>MSLSIPTIKQVRAFVLRGGGADYHDQGDGHWIDDHISTPMGKYPEYRQSRRSFGINVLGTLVVEIEASDGNVGFAVTTGGEPAAYIVEKHLARFLEGARVTDIER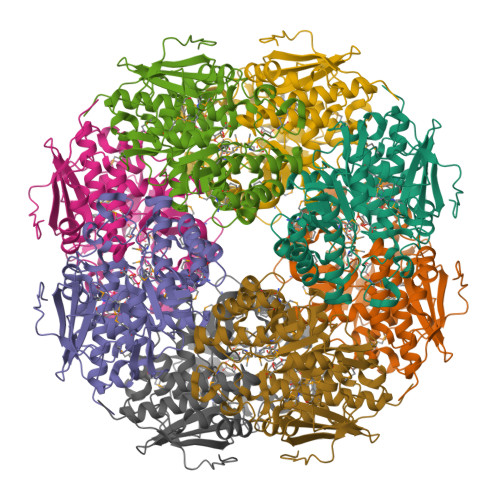IWDQMYNSTLYYGRKGLVINTISGVDLALWDLLGKVRREPVHQLLGGAVRDELQFYATGARPDLAQKMGFIGGKMPLHHGPSEGEEGLKKNLEELATMRERVGPDFWLMFDCWMSLDLNYATRLARGAREYGLKWIEEALPPDDYWGYAELRRNAPTGMMVTTGEHEATRWGFRMLLEMGCCDIIQPDVGWCGGVTELLKISALADAHNALVVPHGSSVYSYHFVATRQNSPFAEFLMMAPKADQVVPMFHPQLLGEPVPENGRMRLSRLDQPGFGVTLNPECQLHRPYTHEGHHHHHH[2x]>[2x]MTMDEQQSQAVAPVYVGGFLARYDQSPDEAELLLPRDVVEHWLHAQGQGQPSLSVALPLNINHDDTAVVGHVAAMQSVRDGLFCLGCVTSPRFLEIVRRASEKSELVSRGPVSPLQPDKVVEFLSGSYAGLSLSSRRCDDVEQATSLSGSETTPFKEVALCSVGRRRGTLAVYGRDPEWVTQRFPDLTAADRDGLRAQWQRCGSTAVDASG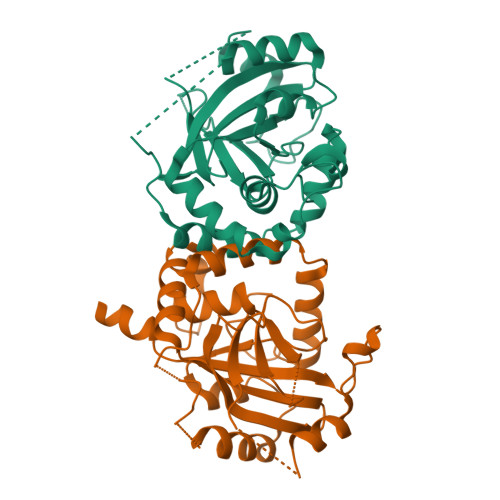DPFRSDSYGLLGNSVDALYIRERLPKLRYDKQLVGVTERESYVKA>TAPSQVLKIRRPDDWHLHLRDGDMLKTVVPYTSEIYGRAIVMPNLAPPVTTVEAAVAYRQRILDAVPAGHDFTPLMTCYLTDSLDPNELERGFNEGVFTAAKLYPANAATNSSHGVTSVDAIMPVLERMEKIGMPLLVHGEVTHADIDIFDREARFIESVMEPLRQRLTALKVVFEHITTKDAADYVRDGNERLAATITPQHLMFNRNHMLVGGVRPHLYCLPILKRNIHQQALRELVASGFNRVFLGTDSAPHARHRKESSCGCAGCFNAPTALGSYATVFEEMNALQHFEAFCSVNGPQFYGLPVNDTFIELVREEQQVAESIALTDDTLVPFL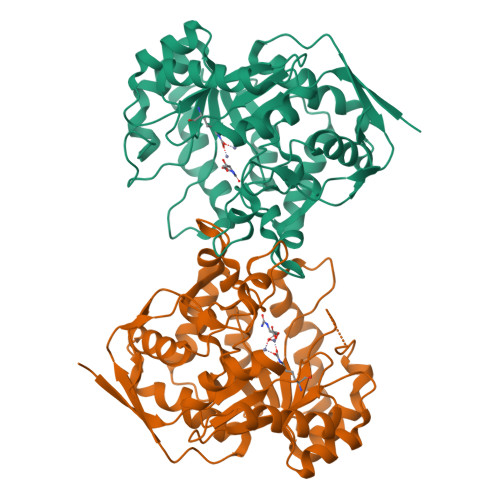AGETVRWSVKQ[2x]>[4x]MVYQVKDQEDFTKQLNEAGNKLVVIDFYATWCGPCKMIAPK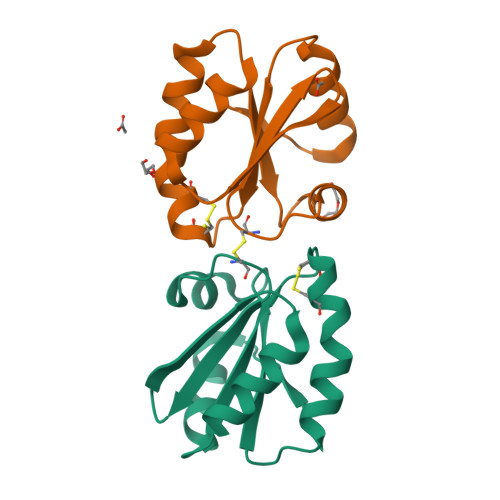LEELSQSMSDVVFLKVDVSECEDIAQDNQIACMPTFLFMKNGQKLDSLSGANYDKLLELVEKNK> ERVNVNLTSIKKLREKVDDSIHRELTDIFANLNYVGVVD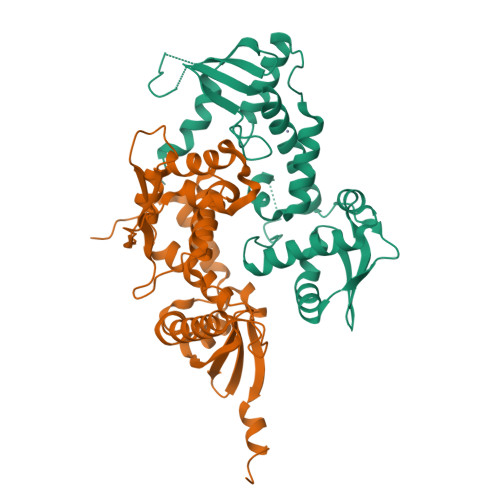EERRLAAIQHDLKLFLIDYGSVCYELFYQIGLTDFANFGKINLQSTNVSDDIVLYNLLSEFDELNDDASKEKIISKIWDMSSMLNEYYSIELVNDGLDNDLKSVKLKSLPLLLKGYIPSLVKLPFFIYRLGKEVDWEDEQECLDGILREIALLYIPDMVPKVDTSDASLSEDEKAQFINRKEHISSLLEHVLFPCIKRRFLAPRHILKDVVEIANLPDLYKVFERC;> GKTITDFSISRSVLAKYEVINQVDKKFILIRCLDQSIHNCPLLVLVDQHACDERIRLEELFYSLLTEVVTGTFVARDLKDCCIEVDRTEADLFKHYQSEFKKWGIGYETIEGTMETSLLEIKTLPEMLTSKYNGDKDYLKMVLLQHAHDLKDFKKLPMDLSHFENYTSVDKLYWWKYSSCVPTVFHEILNSKACRSAVMFGDELTRQECIILISKLSRCHNPFECAHGRPSMVPIAELK N-methyl-N-(4-{(1S)-2,2,2-trifluoro-1-hydroxy-1-[1-(2-methoxyethyl)-1H-pyrrol-2-yl]ethyl}phenyl)benzenesulfonamide 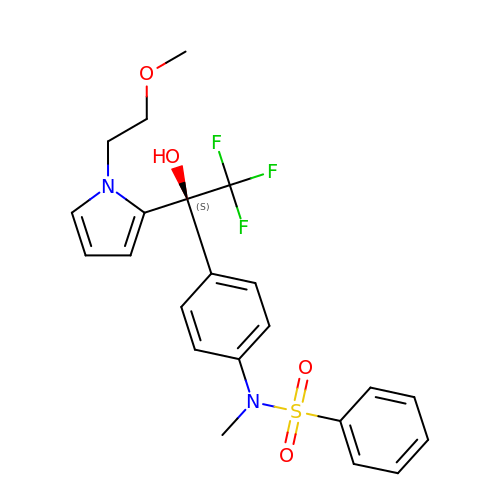| C22 H23 F3 N2 O4 S | YNUCWQDMZHYFEC-NRFANRHFSA-N The C1q molecule is a complex defense collagen, being assembled from six heterotrimeric subunits, each consisting of three homologous, yet distinct polypeptide chains (A–C) encoded by the C1QA, C1QB, and C1QC genes oriented in the A–C–B order on human chromosome 1p. C1q also features the most versatile recognition properties, being able to identify not only bacterial and viral pathogens, either directly or through other immune proteins such as antibodies and pentraxins, but also many altered self elements, including β-amyloid fibrils, the pathological form of the prion protein, modified low-density lipoproteins, and apoptotic cells. We report here, the production of a single-chain recombinant form of human C1q globular region (C1q-scGR). The three monomers have been linked in tandem to generate a single continuous polypeptide, based on a strategy previously used to generate a single-chain form of the homotrimeric globular domain of adiponectin, a protein structurally related to C1q.

Although sialidase treatment of serum-derived C1q-GR had been required to obtain crystals of this protein suitable for structure determination, the presence of sialic acids in C1q-scGR was not an obstacle to the determination of its crystal structure. Its X-ray structure, refined at 1.35 Å resolution, allowed us to check that the linkers did not introduce any distortion. The recombinant and serum-derived C1q globular domains are indeed almost identical, as shown by their very small 0.1 Å RMS deviation on the 331 Cα common positions. The main-chain trace of the segment encompassing the C–B linker and the first two residues of gC1qB (GSAKA) were modeled into the electron density. This more rigid C–B linker only slightly alters the main-chain position of the two preceding and following residues, but the positions of their side-chains are conserved. The A–C linker is more flexible, and only the first two residues of gC1qC were modeled into the electron density. The single N-glysosylation site at Asn 124 of C1qA is thus glycosylated in recombinant C1q-scGR. With a RMS deviation of 0.08 Å on the 340 Cα common positions, the two refined structures are almost identical except for the nature of the bound ion, which is either magnesium or calcium. The presence of a single calcium (or magnesium) ion at the top of the heterotrimeric assembly has been proposed to contribute to the stability of the recognition domain of C1q. The fact that the 3D structure of C1q-scGR is virtually identical to that of the three-chain C1q-derived fragment shows that this strategy can be extended to other proteins containing trimeric gC1q domains.

> KDQPRPAFSAIRRNPPMGGNVVIFDTVITNQEEPYQNHSGRFVCTVPGYYYFTFQVLSQWEICLSIVSSSRGQVRRSLGFCDTTNKGLFQVVSGGMVLQLQQGDQVWVEKDPKKGHIYQGSEADSVFSGFLIFPSAGSGKQKFQSVFTVTRQTHQPPAPNSLIRFNAVLTNPQGDYDTSTGKFTCKVPGLYYFVYHASHTANLCVLLYRSGVKVVTFCGHTSKTNQVNSGGVLLRLQVGEEVWLAVNDYYDMVGIQGSDSVFSGFLLFPDGSAKATQKIAFSATRTINVPLRRDQTIRFDHVITNMNNNYEPRSGKFTCKVPGLYYFTYHASSRGNLCVNLMRGRERAQKVVTFCDYAYNTFQVTTGGMVLKLEQGENVFLQATDKNSLLGMEGANSIFSGFLLFPDMEA> TFISRFAPDQPRKGADILVEALERQGVETVFAYPGGASMEIHQALTRSSSIRNVLPRHEQGGVFAAEGYARSSGKPGICIATSGPGATNLVSGLADALLDSVPLVAITGQVPRRMIGTDAFQETPIVEVTRSITKHNYLVMDVEDIPRIIEEAFFLATSGRPGPVLVDVPKDIQQQLAIPNWEQAMRLPGYMSRMPKPPEDSHLEQIVRLISESKKPVLYVGGGCLNSSDELGRFVELTGIPVASTLMGLGSYPCDDELSLHMLGMHGTVY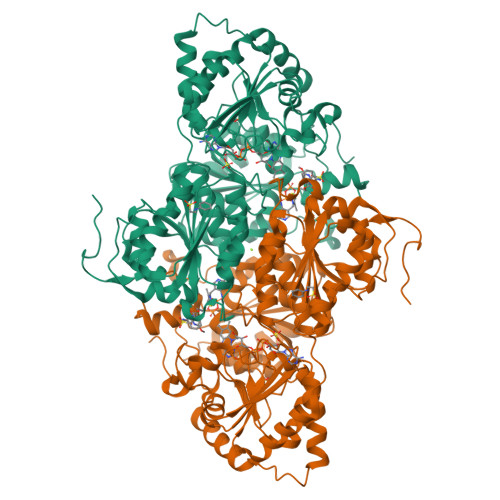ANYAVEHSDLLLAFGVRFDDRVTGKLEAFASRAKIVHIDIDSAEIGKNKTPHVSVCGDVKLALQGMNKVLENRAEELKLDFGVWRNELNVQKQKFPLSFKTFGEAIPPQYAIKVLDELTDGKAIISTGVGQHQMWAAQFYNYKKPRQWLSSGGLGAMGFGLPAAIGASVANPDAIVVDIDGDGSFIMNVQELATIRVENLPVKVLLLNNQHLGMVMQLEDRFYKANRAHTFLGDPAQEDEIFPNMLLFAAACGIPAARVTKKADLREAIQTMLDTPGPYLLDVICPHQEHVLPMIPSGGTFNDVITEGDGRLEHHHHHH> GSHMSLSKQVVPTHRVEIAPNSESTAKMDHSNYQHNGLITKIWGTAGWTFNHAVTFGYPLNPTSDDKRRYKNYFISLGDVLPCRLCRESYKKFITTGKTALTNEVLRNRHTLTKWFYDVHNAVNNKLEVDYGLSYEDVVNKYESFRAKCGKPVPTVKGCVTPLDHKAFSFKKLYYMDAPIVSLDKVENFVRIARM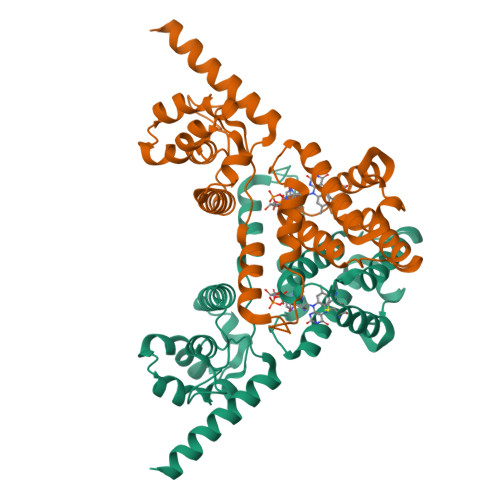RGISDKYFAFLELATVLNGDFNELKKQSSWEYRNKYAQKKIRHMRENAIPSIEEQGYWKGTPTIDELKLLLFLASNLNRTEVNDAINNVERLESTHYIEN N-{[(2E)-2-{[4-(trifluoromethyl)phenyl]methylidene}hydrazino]carbonothioyl}-beta-D-glucopyranosylamine 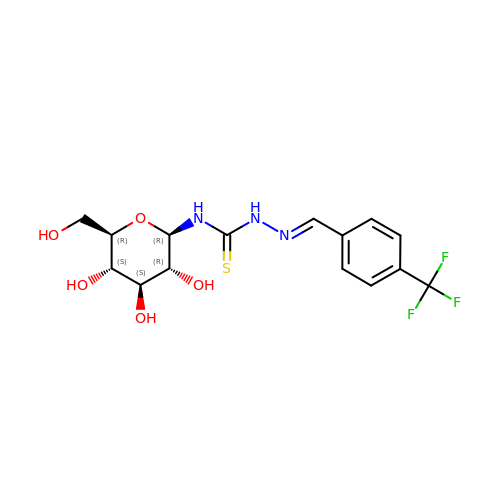| C15 H18 F3 N3 O5 S | SPEHXGJLVCNQJH-HORNZCGOSA-N>[36x]XVQSKI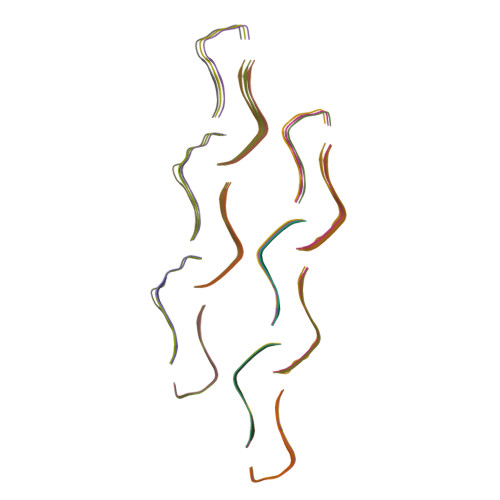GSLDNITHX>[4x]MAHHHHHHHRSADQETEPGVPADLPAESDPAALERLAARYRRDGYVHVPGVLDAGEVAEYLAEARRLLAHEESVRWGSGAGTVMDYVADAQLGSDTMRRLATHPRIAALAEYLAGSPLRLFKLEVLLKENKEKDASVPTAPHHDAFAFPFSTAGTALTAWVALVD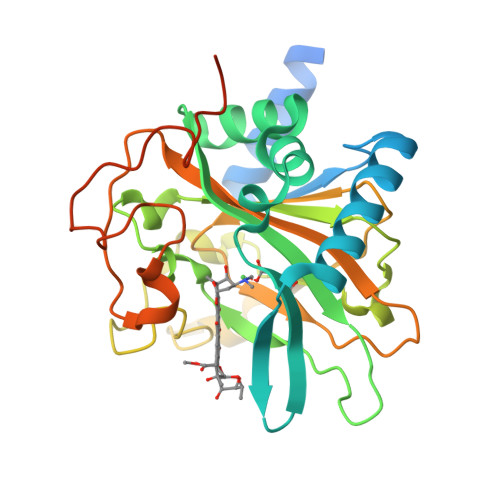VPVERGCMTFVPGSHLLPDPDTGDEPWAGAFTRPGEIWMPRVTVPLRAGDCTFHHARTVHSAGANSTDEPRLSTSAVYMDATAAYRPTGIAFLDDLPGTGADPLREGAPLTGDRFPLLRRPQTRQPAPARYPLPQQGHGS>MTPLETVQLFLARVNALDLDGACALLAEDVVYDNVPMPTVHGRAAARAFLS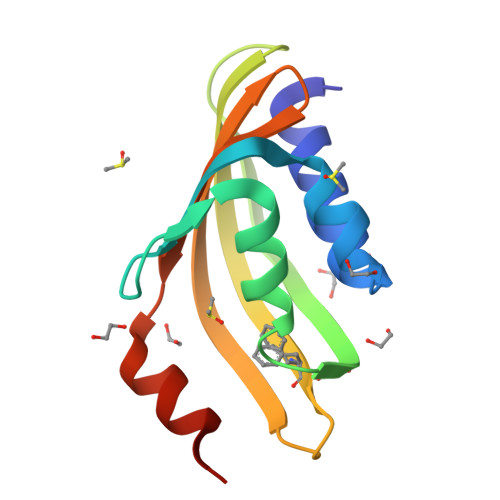QLPATAIDWETHAIAATGDAARGTVLTERTDRFTLADGRTLAIRVMGAFDVADGSITAWRDYFDLGQFMAQMAPSPSA[2x]> SMMELRVGNRYRLGRKIGSGSFGDIYLGTDIAAGEEVAIKLECVKTKHPQLHIESKIYKMMQGGVGIPTIRWCGAEGDYNVMVMELLGPSLEDLFNFCSRKFSLKTVLLLA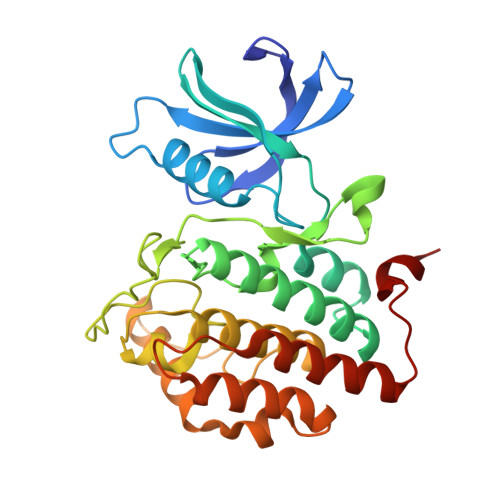DQMISRIEYIHSKNFIHRDVKPDNFLMGLGKKGNLVYIIDFGLAKKYRDARTHQHIPYRENKNLTGTARYASINTHLGIEQSRRDDLESLGYVLMYFNLGSLPWQGLKAATKRQKYERISEKKMSTPIEVLCKGYPSEFATYLNFCRSLRFDDKPDYSYLRQLFRNLFHRQGFSYDYVFDWNMLK>[2x]GSFLLPKLTSKKEVDQAIKSTAEKVLVLRFGRDEDPVCLQLDDILSKTSSDLSKMAAIYLVDVDQTAVYTQYFDISYIPSTVFFFNG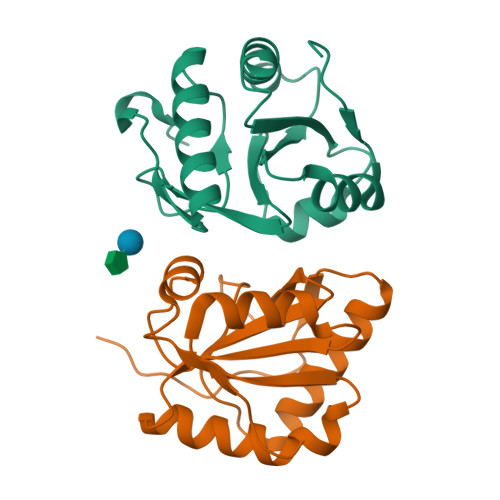QHMKVDYGSPDHTKFVGSFKTKQDFIDLIEVIYRGAMRGKLIVQSPIDPKNIPKYDLLYQDI>GAMATLLEKTRQVNELLQKNN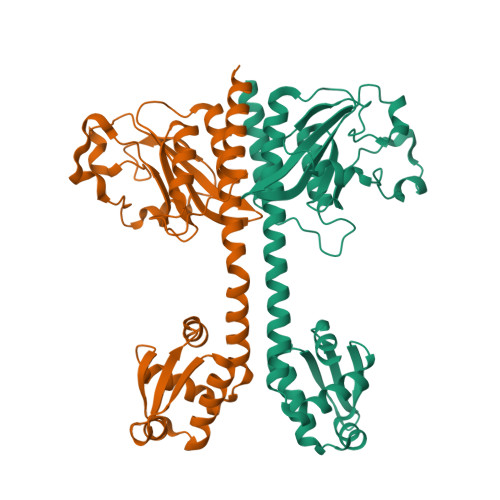LFDVQAELPYNKMAMILGDILESNAYIISSSGDLLGYTEKLDVNNARIKNMFKEKKFPQGYTEAVDMLKVTEANIPIDSDLTAFPFESRELYPFGLTTIVPLYGAGKRLGTIILARVEKSFNEDDLVLAEYSATVVGMQILYHQSRTIEAEVRSATAVQMAINTLSYSELKAVHAIFEALDGEEGRLTASSIADEIGITRSVIVNALRKLESAGIIESRSLGMKGTYLKVLNQQFIKELEK[4x]> AQDNSRYTHFLTQHYDAKPQGRDDR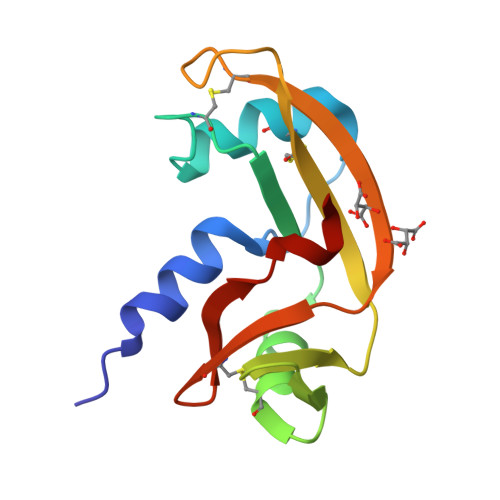YCESIMRRRGLTSPCKDINTFIHGNKRSIKAICENKNGNPHRENLRISKSSFQVTTCKLHGGSPWPPCQYRATAGFRNVVVACENGLPVHLDQSIFRRP> GCDDNDGYSLGDIAVDWATVRVVGGDTYSLNADRWGTLWPAATAIPFYKPIDGQRVITYFNPLYDNYEGYDHAVKVEHNYNVLTKQVEDLTAENESEFGNDPVWVNKDMMWIGGGYLNVIFRQNLPVKEKHLVSLVRDMRATAAEGEDDGYIHLELRYKTYDDVTARQANGAVSFNLNSLDLTGKKGIKVKLNSVKDGETEVVFNLKGQSMPEEAKQVTLSDE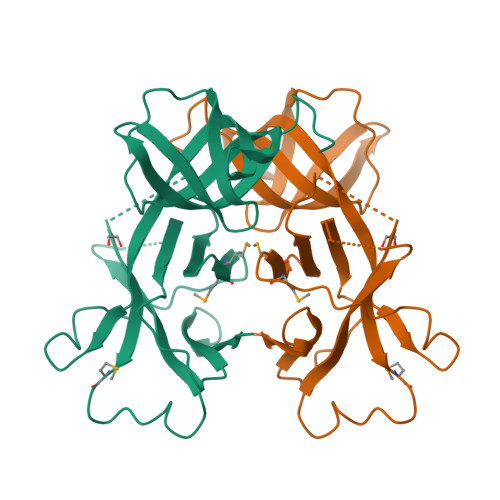VQIK>[4x]HHHHHHAENAGIYGSQSRDD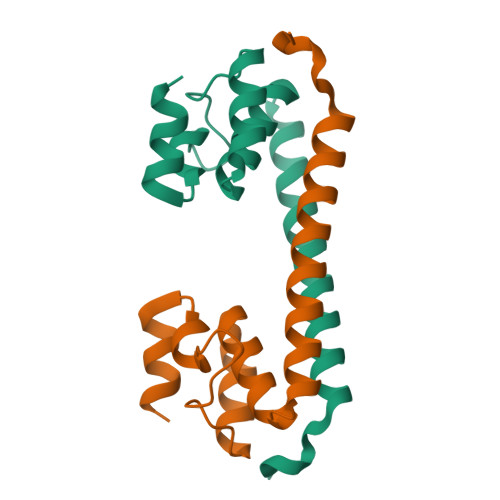FDRDDVEQYFNYMGMLAVEGTYSKMEALLNLNIHPVDILLMLAATEGDRPKIEELLKAGADYSVKDADGRTAIDRANSEEIRDLILGYSTQKA> MGMWKWLVIASLVWPALSLRNVYDMKIECPHTVSFGENSVIGYVELPPMPLADTAQMVPESSCSMDNHQSINTITKYTQVIWRGKADPGQSSQNSFETVSTEVDLKGTCVLKHKMVEESYRSRKSITCYDLSCNSTFCKPTLYMIVPIHACNMMKSCLIALGPYRVQVVYERTYCMTGVLIEGKCFVPDQSVVSIIKHGIFDIASVHVVCFFVAVKGNTYKLFEQVKKSFEST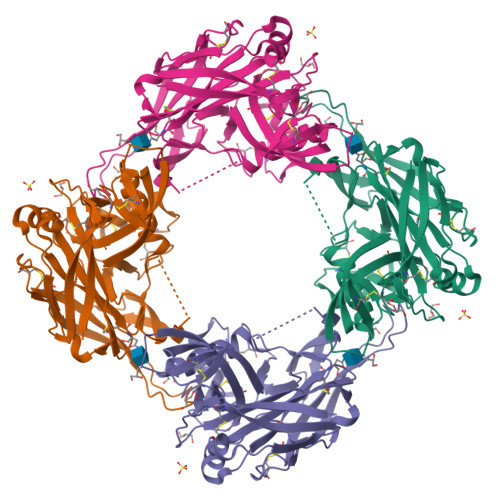CNDTENKVQGYYICIVGGNSAPIYVPTLDDFRSMEAFTGIFKSPHGEDHDLAGEEIASYSIVGPANAKVPHSASSDTLSLIAYSGIPSYSSLSILTSSTDAKHVFSPGLFPKLNHTNCDKSAIPLTWTGMIDLPGYYE>MSQQPGVLPENMKRYMGRDAQRMNILAGRIIAETVRSTLGPKGMDKMLVDDLGDVVVTNDGVTILREMSVEHPAAKMLIEVAKTQEKEVGDGTTTAVVVAGELLRKAEELLDQNVHPTIVVKGYQAAAQKAQELLKTIACEVGAQDKEILTKIAMTSITGKGAEKAKEKLAEIIVEAVSAVVDDEGKVDKDLIKIEKKSGASIDDTELIKGVLVDKERVSAQMPKKVTDAKIALLNCAIEIKETETDAEIRITDPAKLMEFIEQEEKMLKDMVAEIKASGANVLFCQKGIDDLAQHYLAKEGIVAARRVKKSDMEKLAKATGANVITNIKDLSAQDLGDAGLV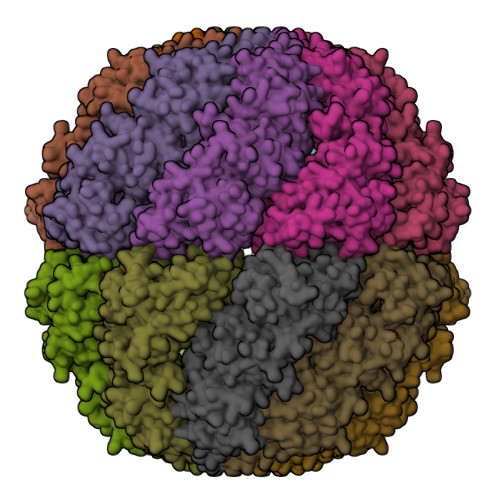EERKISGDSMIFVEECKHPKAVTMLIRGTTEHVIEEVARAVDDAVGVVGCTIEDGRIVSGGGSTEVELSMKLREYAEGISGREQLAVRAFADALEVIPRTLAENAGLDAIEILVKVRAAHASNGNKCAGLNVFTGAVEDMCENGVVEPLRVKTQAIQSAAESTEMLLRIDDVIAAEKLRGAPDMGDMGG[16x]> MAAPARDPPGYRYAAAILPTGSILSTIEVASHRRLFDFFAAVRSDENSLYDVEFDALLGSYCNTLSLVRFLELGLSVACVCTKFPELAYMNEGRVQFEVHQPLIARDGPHPVEQPVHNYMTKVIDRRALNAAFSLATEAIALLTGEALDGTGISLHRQLRAIQQLARNVQAVLGAFERGTADQMLHVLLEKAPPLALLLPMQRYLDNGRLATRVARATLVAELKRSFCDTSFFLGKAGHRREAIEAWLVDLTTATQPSVAVPRLTHADTRGRPVDGVLVTTAAIKQRLLQSFLKVEDTEADVPVTYGEMVLNGANLVTALVMGKAVRSLDDVGRHLLDMQEEQLEANRETLDELESAPQTTRVRADLVAIGDRLVFLEALERRIYAATNVPYPLVGAMDLTFVLPLGLFNPAMERFAAHAGDLVPAPGHPEPRAFPPRQLFFWGKDHQVLRLSMENAVGTVCHPSLMNIDAAVGGVNHDPVEAANPYGAYVAAPAGPGADMQQRFLNAWRQRLAHGRVRWVAECQMTAEQFMQPDNANLALELHPAFDFFAGVADVELPGGEVPPAGPGAIQATWRVVNGNLPLALCPVAFRDARGLELGVGRHAMAPATIAAVRGAFEDRSYPAVFYLLQAAIHGNEHVFCALARLVTQCITSYWNNTRCAAFVNDYSL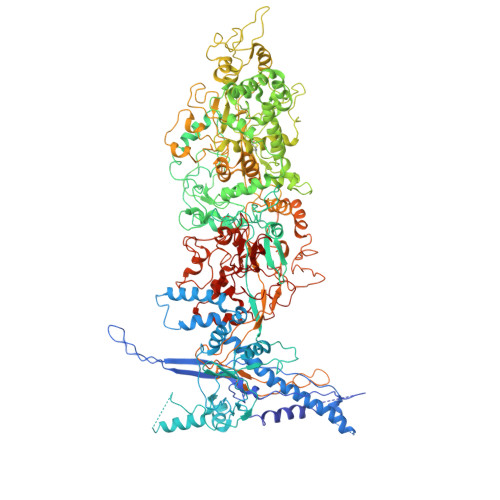VSYIVTYLGGDLPEECMAVYRDLVAHVEALAQLVDDFTLPGPELGGQAQAELNHLMRDPALLPPLVWDCDGLMRHAALDRHRDCRIDAGGHEPVYAAACNVATADFNRNDGRLLHNTQARAADAADDRPHRPADWTVHHKIYYYVLVPAFSRGRCCTAGVRFDRVYATLQNMVVPEIAPGEECPSDPVTDPAHPLHPANLVANTVKRMFHNGRVVVDGPAMLTLQVLAHNMAERTTALLCSAAPDAGANTASTANMRIFDGALHAGVLLMAPQHLDHTIQNGEYFYVLPVHALFAGADHVANAPNFPPALRDLARDVPLVPPALGANYFSSIRQPVVQHARESAAGENALTYALMAGYFKMSPVALYHQLKTGLHPGFGFTVVRQDRFVTENVLFSERASEAYFLGQLQVARHETGGGVNFTLTQPRGNVDLGVGYTAVAATGTVRNPVTDMGNLPQNFYLGRGAPPLLDNAAAVYLRNAVVAGNRLGPAQPLPVFGCAQVPRRAGMDHGQDAVCEFIATPVATDINYFRRPCNPRGRAAGGVYAGDKEGDVIALMYDHGQSDPARPFAATANPWASQRFSYGDLLYNGAYHLNGASPVLSPCFKFFTAADITAKHRCLERLIVETGSAVSTATAASDVQFKRPPGCRELVEDPCGLFQEAYPITCASDPALLRSARDGEAHARETHFTQYLIYDASPLKGLSL> SNMWVIGKSKAQDAKAIMVNGPQFGWYAPAYTYGIGLHGAGYDVTGNTPFAYPGLVFGHNGVISWGSTAGFGDDVDIFAERLSAEKPGYYLHNGKWVKMLSREETITVKNGQAETFTVWRTVHGNILQTDQTTQTAYAKSRAWDGKEVASLLAWTHQMKAKNWQQWTQQAAKQALTINWYYADVNGNIGYVHTGAYPDRQSGHDPRLPVPGTGKWDWKGLLPFEMNPKVYNPQSGYIANWNNSPQKDYPASDLFAFLWGGADRVTEIDRLLEQKPRLTADQAWDVIRQTSRQDLNLRLF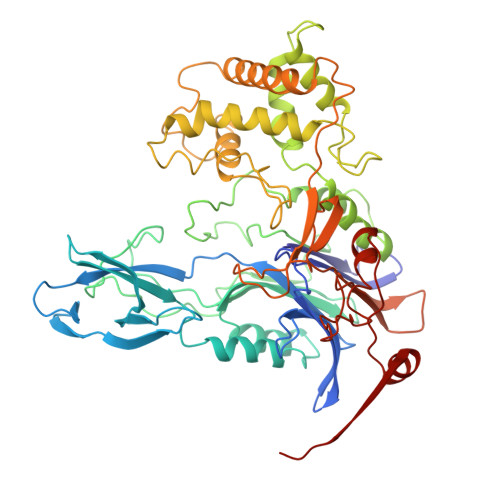LPTLQAATSGLTQSDPRRQLVETLTRWDGINLLNDDGKTWQQPGSAILNVWLTSMLKRTVVAAVPMPFDKWYSASGYETTQDGPTGSLNISVGAKILYEAVQGDKSPIPQAVDLFAGKPQQEVVLAALEDTWETLSKRYGNNVSNWKTPAMALTFRANNFFGVPQAAAEETRHQAEYQNRGTENDMIVFSPTTSDRPVLAWDVVAPGQSGFIAPDGTVDKHYEDQLKMYENFGRKSLWLTKQDVEAHKESQEVLHVQR> SNASVYDPAATADTVNPGNKIIYLTFDDGPGKYTQGLLDVLDK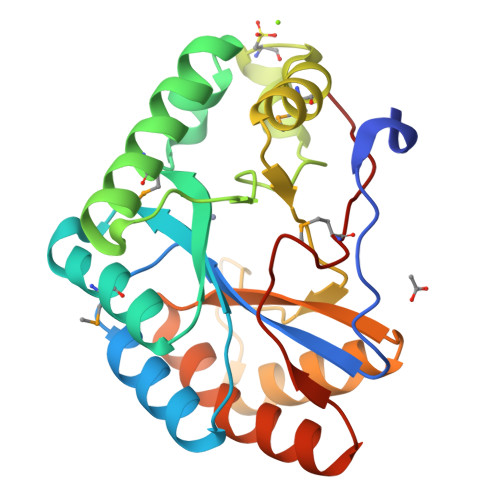YNVKATFFVTNTHPDYQNMIAEEAKRGHTVAIHSASHKYNQIYTSEQAFFDDLEQMNSIIKAQTGNDASIIRFPGGSSNTVSKDYCPGIMTQLVNDVTARGLLYCDWNVSSGDANPKPISTEQVVQNVISGVQSHNVSVVLQHDIKEFSVNAVEQIIQWGQANGYTFLPLTTSSPMSHHRVNN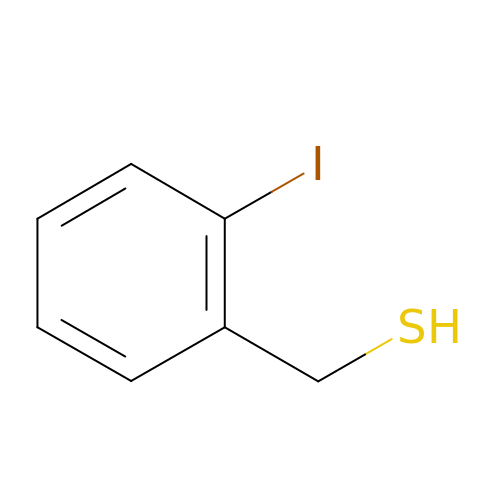2-IODOBENZYLTHIO GROUP | C7 H7 I S | KVYARXTXGITUCU-UHFFFAOYSA-N>[2x]SEGWQFVQENGRTYYKKGDLKETYWRVIDGKYYYFDSLSGEMVVGWQYIPFPSKGSTIGPYPNGIRLEGFPKSEWYYFDKNGVLQEFVGWKTLEIKTKDSVGRKYGEKREDSEDKEEKRYYTNYYFNQNHSLETGWLYDQSNWYYLAKTEINGENYLGGERRAGWINDDSTWYYLDPTTGIMQTGWQYLGNKWYYLRSSGAMATGWYQEGTTWYYLDHPNGDMKTGWQNLGNKWYYLR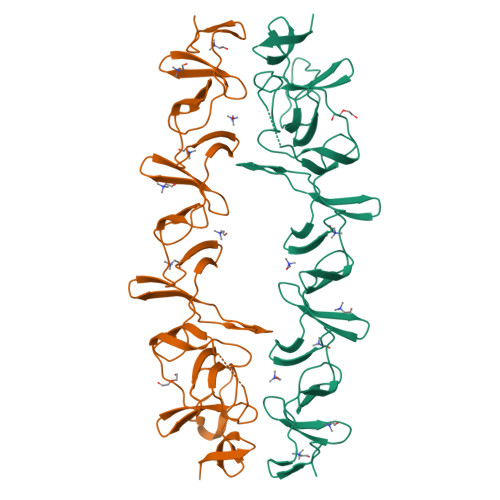SSGAMATGWYQDGSTWYYLNAGNGDMKTGWFQVNGNWYYAYSSGALAVNTTVDGYSVNYNGEWVR2-[CARBOXY-(2-THIOPHEN-2-YL-ACETYLAMINO)-METHYL]-5-METHYLENE-5,6-DIHYDRO-2H-[1,3]THIAZINE-4-CARBOXYLIC ACID | C14 H14 N2 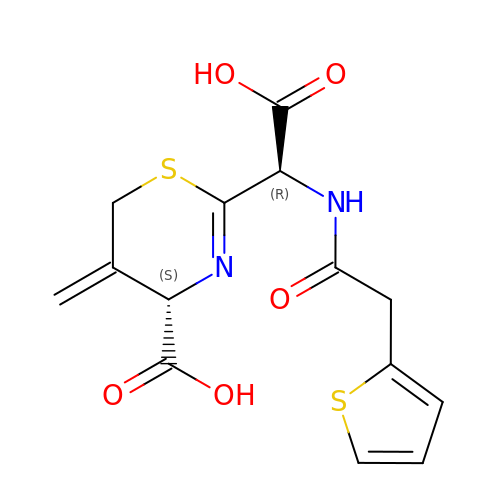O5 S2 | VBBNCGUNWSPHOY-QWRGUYRKSA-N>DLSKHPSGIVPTLQNIVSTVNLDCKLDLKAIALQARNAEYNPKRFAAVIMRIREPKTTALIFASGKMVCTGAKSEDFSKMAARKYARIVQKLGFPAKFKDFKIQNIVGSCDVKFPIRLEGLAYSHAAFSSYEPELFPGLIYRMKVPKIVLLIFVSGKIVITGAKMRDETYKAFENIYPV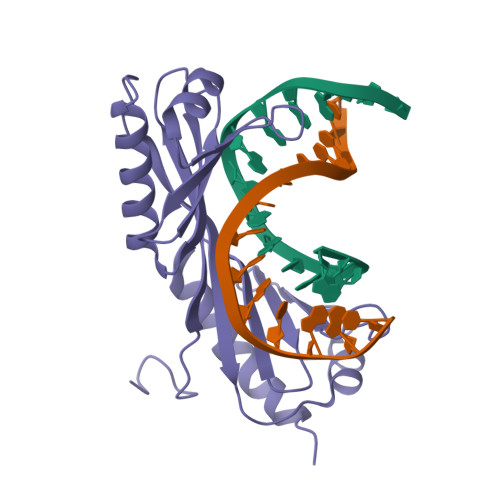LSEFRKI[2x]>MKSQSIMSVERSAETSLTLEIPTSPLIIKITQQERNILSNVGNLLVKAFGNYENPDYIASLHLHAFQLLPERITRILSQFGSDFSAEQYGAIVFQGLIEVDQDDLGPTPPNWQGADYGKLNKYGFICSLLHGAVPSKPVQYYAQRKGGGLLHAVIPDEKMAATQTGSGSKTDLFVHTEDAFLSNQADFLSFLYLRNEERVPSTLYSIRSHGKMNPVMKKLFEPIYQCPKDANYNDEDVANSGPTASVLYGNRELPFIRFDAAEQIFNENAGQTSEALGNLMDFWDEAKTLINSDYIPNSGDLIFVNNHLCAHGRSAFIAGQRIENGEIIKCERRQMLRMMSKTSLIHIRSVTRTDDPYFIM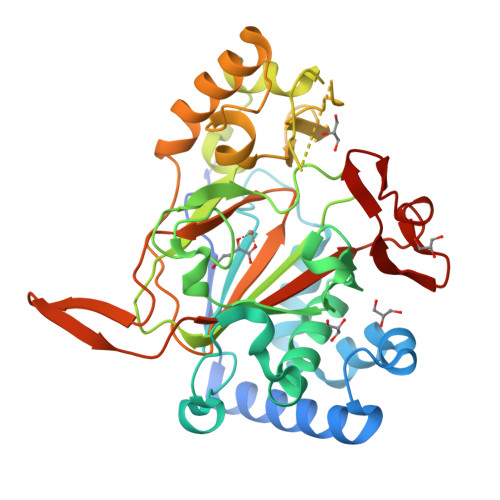EEHLGKIFDLD[4x]>MADFSLATASQRKEWSNKAHM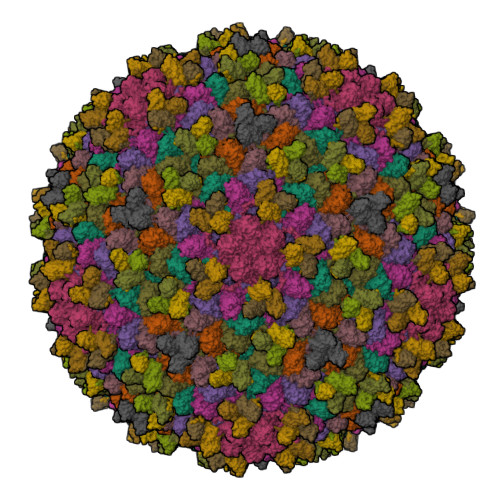EYVRRSRFAPYIRNTENSIFQGYSDLEKRAGDTLNIPLFYKLGGAPVTGDTPIVGNETPLDNYNCGVPVALRGKGVAITKNQTFRTEIDVMNAAKQSLTRYFGELLRDDIIEALGSVVTTGDTTVNYGSASAANRNAFSAANPDRLFFGSISGYSATWATGLGNVDAAETCTAARVGVMKRLAMSASPAITPMQVDDDEGREYFVAFHGSRTFRDLKGDTAMLNANREARPRDVSSNPLLQDGDLIYEGVIHREVPEIDAWAAANGFNTAGAGSAPIRPVFLCGTQSVFLAYAQRPQAGTEKSDIPALNRRMTVGMDEIIGVKKAAFNGKQHGVVMGFFGAAGD[7x];>MPATNSAQARLAAPGHGFGGNVKVSYGSVAFTGTITTADAATVCNLPVGAIVLGVTLESDDLDTNATPTITLNVGDAGSATRYFSASTVAQAGTSSSAPATTGLLWTVTEGNTAVRIAVANNAATSADGSVRVAVTYYLP[7x]Here, we present a tagging strategy for cryoET that precisely identifies individual protein complexes in tomograms without relying on metal clusters. Our method makes use of DNA origami to produce “molecular signposts” that target molecules of interest, here via fluorescent fusion proteins, providing a platform generally applicable to biological surfaces. We have used DNA origami to construct a “signpost” structure, where the “sign” provides the signal for identification in cryoEM images and the bottom of the post is linked to an RNA aptamer that targets common fluorescent proteins (Shui et al., 2012). The signpost origami tags (SPOTs) are used to identify the proteins of interest in a 3D volume of the sample generated by cryoET.

We designed the signpost tags by using the DNA origami method, which enables robust assembly of large and complex nanostructures. In this technique, a long “scaffold” strand is folded into a designed shape through hybridization to many complementary “staple” strands. The signpost is built from a 7,249-nucleotide scaffold strand (single-stranded M13mp18) hybridized to 238 staple oligonucleotides to form a structure of approximately 5 MDa comprising 96 parallel helices arranged in a honeycomb lattice. Signpost origami nanostructures were folded by thermal annealing and purified by polyethylene glycol (PEG) precipitation followed by molecular weight cut-off filtration (full protocols provided in STAR methods). Five mM Mg2+ was maintained in all subsequent preparations to retain proper folding of the nanostructures. The structure of the signpost origami was first verified by negative-stain electron microscopy. Nanostructures were subsequently imaged in vitrified cell lysate by cryoEM to confirm that the contrast of the structure was sufficient to allow it to be identified in crowded biological environments. In projection images, SPOTs are easily identified by the contrast of the repeating stripe patterns generated by the overlap of aligned DNA helices. In tomograms, details to the level of individual DNA helices were visible and the overall shape of the SPOTs was clearly recognizable, and there was sufficient contrast to orient the sub-volume averaging structure by eye. SPOTs have higher contrast than the surrounding protein and often lipids as a result of the phosphorus in the aligned DNA backbones.

> TAAGTACAACCACAGCATTCCAGAACACGTCAACAAATAAGGAACAAAACTCGTATT;> AAGCCAGAATGCCCTTTTAACTGAGGTTTAA;> TCATAACCCGTCGGATGTAGATG;> CAGAGGCCCATCAATATGAGTTTTTATA;> TTGTATCGGATTTTCATAGTTAGCGTAAACCCTCATAGGTGT;> GGAAGCAAACTCCATTGAGTTAAGCC;> TCAGATGATGGCAATTATCATATTTACAAAGTCTTTC;> GAGTAGATTTAGATAACCTGTTTA;> TTTTTGAGAGATATTTAGG;> CATCACGCAAATGCCGGAGAAGG;> ATATATCGGTTATGCGTGGGCGATGGTTGTTGTCATTGTCGGCGCAACTATCGGTATCAAGCTGTTTAAGAAATTCACCTCGAAAGCAAGCTGATAAACCGATACAATTAAAGGCTCCTTTTGGAGCCTTTTTTTTGGAGATTTTCAACGTGAAAAAATTATTATTCGCAATTCCTTTAGTTGTTCCTTTCTATTCTCACTCCGCTGAAACTGTTGAAAGTTGTTTAGCAAAATCCCATACAGAAAATTCATTTACTAACGTCTGGAAAGACGACAAAACTTTAGATCGTTACGCTAACTATGAGGGCTGTCTGTGGAATGCTACAGGCGTTGTAGTTTGTACTGGTGACGAAACTCAGTGTTACGGTACATGGGTTCCTATTGGGCTTGCTATCCCTGAAAATGAGGGTGGTGGCTCTGAGGGTGGCGGTTCTGAGGGTGGCGGTTCTGAGGGTGGCGGTACTAAACCTCCTGAGTACGGTGATACACCTATTCCGGGCTATACTTATATCAACCCTCTCGACGGCACTTATCCGCCTGGTACTGAGCAAAACCCCGCTAATCCTAATCCTTCTCTTGAGGAGTCTCAGCCTCTTAATACTTTCATGTTTCAGAATAATAGGTTCCGAAATAGGCAGGGGGCATTAACTGTTTATACGGGCACTGTTACTCAAGGCACTGACCCCGTTAAAACTTATTACCAGTACACTCCTGTATCATCAAAAGCCATGTATGACGCTTACTGGAACGGTAAATTCAGAGACTGCGCTTTCCATTCTGGCTTTAATGAGGATTTATTTGTTTGTGAATATCAAGGCCAATCGTCTGACCTGCCTCAACCTCCTGTCAATGCTGGCGGCGGCTCTGGTGGTGGTTCTGGTGGCGGCTCTGAGGGTGGTGGCTCTGAGGGTGGCGGTTCTGAGGGTGGCGGCTCTGAGGGAGGCGGTTCCGGTGGTGGCTCTGGTTCCGGTGATTTTGATTATGAAAAGATGGCAAACGCTAATAAGGGGGCTATGACCGAAAATGCCGATGAAAACGCGCTACAGTCTGACGCTAAAGGCAAACTTGATTCTGTCGCTACTGATTACGGTGCTGCTATCGATGGTTTCATTGGTGACGTTTCCGGCCTTGCTAATGGTAATGGTGCTACTGGTGATTTTGCTGGCTCTAATTCCCAAATGGCTCAAGTCGGTGACGGTGATAATTCACCTTTAATGAATAATTTCCGTCAATATTTACCTTCCCTCCCTCAATCGGTTGAATGTCGCCCTTTTGTCTTTGGCGCTGGTAAACCATATGAATTTTCTATTGATTGTGACAAAATAAACTTATTCCGTGGTGTCTTTGCGTTTCTTTTATATGTTGCCACCTTTATGTATGTATTTTCTACGTTTGCTAACATACTGCGTAATAAGGAGTCTTAATCATGCCAGTTCTTTTGGGTATTCCGTTATTATTGCGTTTCCTCGGTTTCCTTCTGGTAACTTTGTTCGGCTATCTGCTTACTTTTCTTAAAAAGGGCTTCGGTAAGATAGCTATTGCTATTTCATTGTTTCTTGCTCTTATTATTGGGCTTAACTCAATTCTTGTGGGTTATCTCTCTGATATTAGCGCTCAATTACCCTCTGACTTTGTTCAGGGTGTTCAGTTAATTCTCCCGTCTAATGCGCTTCCCTGTTTTTATGTTATTCTCTCTGTAAAGGCTGCTATTTTCATTTTTGACGTTAAACAAAAAATCGTTTCTTATTTGGATTGGGATAAATAATATGGCTGTTTATTTTGTAACTGGCAAATTAGGCTCTGGAAAGACGCTCGTTAGCGTTGGTAAGATTCAGGATAAAATTGTAGCTGGGTGCAAAATAGCAACTAATCTTGATTTAAGGCTTCAAAACCTCCCGCAAGTCGGGAGGTTCGCTAAAACGCCTCGCGTTCTTAGAATACCGGATAAGCCTTCTATATCTGATTTGCTTGCTATTGGGCGCGGTAATGATTCCTACGATGAAAATAAAAACGGCTTGCTTGTTCTCGATGAGTGCGGTACTTGGTTTAATACCCGTTCTTGGAATGATAAGGAAAGACAGCCGATTATTGATTGGTTTCTACATGCTCGTAAATTAGGATGGGATATTATTTTTCTTGTTCAGGACTTATCTATTGTTGATAAACAGGCGCGTTCTGCATTAGCTGAACATGTTGTTTATTGTCGTCGTCTGGACAGAATTACTTTACCTTTTGTCGGTACTTTATATTCTCTTATTACTGGCTCGAAAATGCCTCTGCCTAAATTACATGTTGGCGTTGTTAAATATGGCGATTCTCAATTAAGCCCTACTGTTGAGCGTTGGCTTTATACTGGTAAGAATTTGTATAACGCATATGATACTAAACAGGCTTTTTCTAGTAATTATGATTCCGGTGTTTATTCTTATTTAACGCCTTATTTATCACACGGTCGGTATTTCAAACCATTAAATTTAGGTCAGAAGATGAAATTAACTAAAATATATTTGAAAAAGTTTTCTCGCGTTCTTTGTCTTGCGATTGGATTTGCATCAGCATTTACATATAGTTATATAACCCAACCTAAGCCGGAGGTTAAAAAGGTAGTCTCTCAGACCTATGATTTTGATAAATTCACTATTGACTCTTCTCAGCGTCTTAATCTAAGCTATCGCTATGTTTTCAAGGATTCTAAGGGAAAATTAATTAATAGCGACGATTTACAGAAGCAAGGTTATTCACTCACATATATTGATTTATGTACTGTTTCCATTAAAAAAGGTAATTCAAATGAAATTGTTAAATGTAATTAATTTTGTTTTCTTGATGTTTGTTTCATCATCTTCTTTTGCTCAGGTAATTGAAATGAATAATTCGCCTCTGCGCGATTTTGTAACTTGGTATTCAAAGCAATCAGGCGAATCCGTTATTGTTTCTCCCGATGTAAAAGGTACTGTTACTGTATATTCATCTGACGTTAAACCTGAAAATCTACGCAATTTCTTTATTTCTGTTTTACGTGCAAATAATTTTGATATGGTAGGTTCTAACCCTTCCATTATTCAGAAGTATAATCCAAACAATCAGGATTATATTGATGAATTGCCATCATCTGATAATCAGGAATATGATGATAATTCCGCTCCTTCTGGTGGTTTCTTTGTTCCGCAAAATGATAATGTTACTCAAACTTTTAAAATTAATAACGTTCGGGCAAAGGATTTAATACGAGTTGTCGAATTGTTTGTAAAGTCTAATACTTCTAAATCCTCAAATGTATTATCTATTGACGGCTCTAATCTATTAGTTGTTAGTGCTCCTAAAGATATTTTAGATAACCTTCCTCAATTCCTTTCAACTGTTGATTTGCCAACTGACCAGATATTGATTGAGGGTTTGATATTTGAGGTTCAGCAAGGTGATGCTTTAGATTTTTCATTTGCTGCTGGCTCTCAGCGTGGCACTGTTGCAGGCGGTGTTAATACTGACCGCCTCACCTCTGTTTTATCTTCTGCTGGTGGTTCGTTCGGTATTTTTAATGGCGATGTTTTAGGGCTATCAGTTCGCGCATTAAAGACTAATAGCCATTCAAAAATATTGTCTGTGCCACGTATTCTTACGCTTTCAGGTCAGAAGGGTTCTATCTCTGTTGGCCAGAATGTCCCTTTTATTACTGGTCGTGTGACTGGTGAATCTGCCAATGTAAATAATCCATTTCAGACGATTGAGCGTCAAAATGTAGGTATTTCCATGAGCGTTTTTCCTGTTGCAATGGCTGGCGGTAATATTGTTCTGGATATTACCAGCAAGGCCGATAGTTTGAGTTCTTCTACTCAGGCAAGTGATGTTATTACTAATCAAAGAAGTATTGCTACAACGGTTAATTTGCGTGATGGACAGACTCTTTTACTCGGTGGCCTCACTGATTATAAAAACACTTCTCAGGATTCTGGCGTACCGTTCCTGTCTAAAATCCCTTTAATCGGCCTCCTGTTTAGCTCCCGCTCTGATTCTAACGAGGAAAGCACGTTATACGTGCTCGTCAAAGCAACCATAGTACGCGCCCTGTAGCGGCGCATTAAGCGCGGCGGGTGTGGTGGTTACGCGCAGCGTGACCGCTACACTTGCCAGCGCCCTAGCGCCCGCTCCTTTCGCTTTCTTCCCTTCCTTTCTCGCCACGTTCGCCGGCTTTCCCCGTCAAGCTCTAAATCGGGGGCTCCCTTTAGGGTTCCGATTTAGTGCTTTACGGCACCTCGACCCCAAAAAACTTGATTTGGGTGATGGTTCACGTAGTGGGCCATCGCCTGATAGACGGTTTTTCGCCCTTTGACGTTGGAGTCCACGTTCTTTAATAGTGGACTCTTGTTCCAAACTGGAACAACACTCAACCCTATCTCGGGCTATTCTTTTGATTTATAAGGGATTTTGCCGATTTCGGAACCACCATCAAACAGGATTTTCGCCTGCTGGGGCAAACCAGCGTGGACCGCTTGCTGCAACTCTCTCAGGGCCAGGCGGTGAAGGGCAATCAGCTGTTGCCCGTCTCACTGGTGAAAAGAAAAACCACCCTGGCGCCCAATACGCAAACCGCCTCTCCCCGCGCGTTGGCCGATTCATTAATGCAGCTGGCACGACAGGTTTCCCGACTGGAAAGCGGGCAGTGAGCGCAACGCAATTAATGTGAGTTAGCTCACTCATTAGGCACCCCAGGCTTTACACTTTATGCTTCCGGCTCGTATGTTGTGTGGAATTGTGAGCGGATAACAATTTCACACAGGAAACAGCTATGACCATGATTACGAATTCGAGCTCGGTACCCGGGGATCCTCTAGAGTCGACCTGCAGGCATGCAAGCTTGGCACTGGCCGTCGTTTTACAACGTCGTGACTGGGAAAACCCTGGCGTTACCCAACTTAATCGCCTTGCAGCACATCCCCCTTTCGCCAGCTGGCGTAATAGCGAAGAGGCCCGCACCGATCGCCCTTCCCAACAGTTGCGCAGCCTGAATGGCGAATGGCGCTTTGCCTGGTTTCCGGCACCAGAAGCGGTGCCGGAAAGCTGGCTGGAGTGCGATCTTCCTGAGGCCGATACTGTCGTCGTCCCCTCAAACTGGCAGATGCACGGTTACGATGCGCCCATCTACACCAACGTGACCTATCCCATTACGGTCAATCCGCCGTTTGTTCCCACGGAGAATCCGACGGGTTGTTACTCGCTCACATTTAATGTTGATGAAAGCTGGCTACAGGAAGGCCAGACGCGAATTATTTTTGATGGCGTTCCTATTGGTTAAAAAATGAGCTGATTTAACAAAAATTTAATGCGAATTTTAACAAAATATTAACGTTTACAATTTAAATATTTGCTTATACAATCTTCCTGTTTTTGGGGCTTTTCTGATTATCAACCGGGGTACATATGATTGACATGCTAGTTTTACGATTACCGTTCATCGATTCTCTTGTTTGCTCCAGACTCTCAGGCAATGACCTGATAGCCTTTGTAGATCTCTCAAAAATAGCTACCCTCTCCGGCATTAATTTATCAGCTAGAACGGTTGAATATCATATTGATGGTGATTTGACTGTCTCCGGCCTTTCTCACCCTTTTGAATCTTTACCTACACATTACTCAGGCATTGCATTTAAAATATATGAGGGTTCTAAAAATTTTTATCCTTGCGTTGAAATAAAGGCTTCTCCCGCAAAAGTATTACAGGGTCATAATGTTTTTGGTACAACCGATTTAGCTTTATGCTCTGAGGCTTTATTGCTTAATTTTGCTAATTCTTTGCCTTGCCTGTATGATTTATTGGATGTTAATGCTACTACTATTAGTAGAATTGATGCCACCTTTTCAGCTCGCGCCCCAAATGAAAATATAGCTAAACAGGTTATTGACCATTTGCGAAATGTATCTAATGGTCAAACTAAATCTACTCGTTCGCAGAATTGGGAATCAACTGTTATATGGAATGAAACTTCCAGACACCGTACTTTAGTTGCATATTTAAAACATGTTGAGCTACAGCATTATATTCAGCAATTAAGCTCTAAGCCATCCGCAAAAATGACCTCTTATCAAAAGGAGCAATTAAAGGTACTCTCTAATCCTGACCTGTTGGAGTTTGCTTCCGGTCTGGTTCGCTTTGAAGCTCGAATTAAAACGCGATATTTGAAGTCTTTCGGGCTTCCTCTTAATCTTTTTGATGCAATCCGCTTTGCTTCTGACTATAATAGTCAGGGTAAAGACCTGATTTTTGATTTATGGTCATTCTCGTTTTCTGAACTGTTTAAAGCATTTGAGGGGGATTCAATGAATATTTATGACGATTCCGCAGTATTGGACGCTATCCAGTCTAAACATTTTACTATTACCCCCTCTGGCAAAACTTCTTTTGCAAAAGCCTCTCGCTATTTTGGTTTTTATCGTCGTCTGGTAAACGAGGGTTATGATAGTGTTGCTCTTACTATGCCTCGTAATTCCTTTTGGCGTTATGTATCTGCATTAGTTGAATGTGGTATTCCTAAATCTCAACTGATGAATCTTTCTACCTGTAATAATGTTGTTCCGTTAGTTCGTTTTATTAACGTAGATTTTTCTTCCCAACGTCCTGACTGGTATAATGAGCCAGTTCTTAAAATCGCATAAGGTAATTCACAATGATTAAAGTTGAAATTAAACCATCTCAAGCCCAATTTACTACTCGTTCTGGTGTTTCTCGTCAGGGCAAGCCTTATTCACTGAATGAGCAGCTTTGTTACGTTGATTTGGGTAATGAATATCCGGTTCTTGTCAAGATTACTCTTGATGAAGGTCAGCCAGCCTATGCGCCTGGTCTGTACACCGTTCATCTGTCCTCTTTCAAAGTTGGTCAGTTCGGTTCCCTTATGATTGACCGTCTGCGCCTCGTTCCGGCTAAGTAACATGGAGCAGGTCGCGGATTTCGACACAATTTATCAGGCGATGATACAAATCTCCGTTGTACTTTGTTTCGCGCTTGGTATAATCGCTGGGGGTCAAAGATGAGTGTTTTAGTGTATTCTTTTGCCTCTTTCGTTTTAGGTTGGTGCCTTCGTAGTGGCATTACGTATTTTACCCGTTTAATGGAAACTTCCTCATGAAAAAGTCTTTAGTCCTCAAAGCCTCTGTAGCCGTTGCTACCCTCGTTCCGATGCTGTCTTTCGCTGCTGAGGGTGACGATCCCGCAAAAGCGGCCTTTAACTCCCTGCAAGCCTCAGCGACCGA;> GACAATATTTTTCGCGAG;> TAATCAGTAGCGACATAGTAAGAGCAAGGCTTTGTTTTGC;> GGGTCAGCGATTATAAAGAGGCAAAAGAAACGGCTATCGTCA;> AAACAAATACAGATAGCC;> AGATTAAGATTGGGTTAT;> ATTAATGCCGAGAGTCTG;> TCGCCCAGCAGGGAGACTTTTCAACATTGAAAGATTCA;> CAATAATTGTACAGGAGTAATCTT;> TTACGCCAGTTTCCCAGT;> TACTTTTCATCGTAGGAATCATTTAGT;> ATTGCCTGGAGAGGCCGTTCTGAGAAAGTAACCGTCACTTGCCTGAGTAGAAGA;> GTTCCGAAATCGGCAAATACTTCTTGATGGTG;> CGAGCCGGAAGCATAAAGGAAAGGACCTTGTAAAGCC;> ACGACGATAAAAGTAAAAT;> CCCGTATAAACTTCTTAAGATATTCAC;> GGCTGACCTAACAAAGCT;> ACCGTAATGGGAAGGGGACGA;> TTGAAAATAGAAACAGTACAAACTACAAATAGGAGATAAGTG;> AAGTAAGAATCCTCTGGCCTTACAGCTTCAGCGAAGGAACGAGGG;> AAGTTCTTAATTGTGTCTGGAAGTATTTTGCAC;> ATAGCAAGCATTTTGAAGGAACCAGCCGCCAGACAGGAGCAGTCTGGCTTTTGA;> GGTCCGATGAACGGTAATCGTAAAATT;> TATAATAAAAGAGTCTGTC;> TAGAACCCTTCTCGTAAGAATACGTGGCACA;> CAGAGGGTCACCAGATTTGTATCATC;> CTATTATCCCGGAAGAGCCACCACCCTCCAGCCCTGCTAAAC;> GACAAGAACAGCCGCCGC;> TGGTTCTCCGTTCAAATAAGATTAAGAGGAAGCC;> CGAATAATAATTAGGATTAGC;> GAGCGCTAGAAACAACTGGCACAAACGTAATAGTGCTTTTTAACCT;> TAAGTTGGGTAACGGACGGCC;> TATAGAAGGCTTATAACCTCCACCGCCTCTCAGAGAGACGATATTA;> CAACATGTACTACAAAGGCTAAGGAGGCCG;> ATCAGTGAGGCCACCGAGATCAA;> TGAGCTAACGTGCCAGCT;> CGTCACCAATGAAACCATAAGAATGCAACGATAGCAGCACCG;> TCAAGAGCCAGGCGACCCATGTACCGTAACACT;> CCAGCGGATATTCATTGTCATTTCTTAGAGTGAGTAACCGAAC;> GGCGCATTAATTAACAAAA;> TCGGTCGCTTAGTAAATTGGGCTGAATTAC;> TTAGACGAATAACACGCCACCCCCTCAGAGCCGCCAC;> GTTATTAATTGCGATGCAAGTTAA;> GCTATATTTTCATCTACTATTGCGCTTTTCCAG;> TTAATTGAGAATCGCCCGCTCAATGAATTAATTGACGAGTG;> GTTGAGTGTTGTTCCGCCA;> TCACATTTGGGGTGCCTAATGAG;> TAGCGTCCAATACTGAGCCAATTAGCGGAATCGTCATA;> CGAGATCCCCCTCAAACGAT;> CCACGCCTTTAGCCATATGGAGCGGAGACTTTACA;> CATCTGCAGGAAGAGCGAACCAGACC;> AAGCATCTTTAATCACCGCCTTAACAATTTTTCAATATATATCTTTAG;> GGAAGCGCAACAGTAACA;> AAATATCTAAACTGGTCAGGTCAGTATTA;> CTGCTCATCCGCAAAAAG;> GAGCAAACACGGTTGATA;> GAGAAGTTATTCAAGTAGCTAGTTTAGACTGGA;> AATTGCGATAGTAGTAGCA;> AGCAAAAGGTAATAACCAAAATAAAGTACAGCTAATGCAGAACGCGC;> TACTGGCGACAATCCGTAA;> CCTCAGAACTAAAAACAG;> TCTGTAAATCGTCGCTATCGTAACCGTG;> CCCTCAGGATACCGAGTAACAGTG;> GAGAGTACCTTTAATTGCTATAATGCATGTGCT;> AACAACTAACATATCAAACAACAGTGCCA;> GTGGAGGCAAAGACGTTGGGAAG;> CTTACTTGAGCCATTTGGG;> CGGTACAGTTTGGAACAAG;> TCGGGAACAACGCGTCGGTTGTACCA;> CATTAAAGGCAGTAGGGC;> TGATACAGGGAAATTATT;> GCTCATTCAGATTCCCGCAACTATCGACTCAGTGCCAAGCTTGCATAAAGG;> CCTTGCTTTAGAATCCTTGAAAAGAGTCAGAAAATCGCAAAG;> ACGTTGGTGAATAGTTAATGCCCCCTTACTCAGCCCTCAG;> ATAAGAGACCCAAAAGGCTTGCCCTGACGAGAAAC;> ACATTTGAGGATTTAGGCCG;> TTAAACCAAGTACGAGAACAA;> ATATCATATGGCTGCGCACGGGGAAAGCCGG;> ATTAAAGGGATTTTAGACAGGAAGAATCCT;> CTGGCCACCCGCCACTGACAGAGA;> AATATTCATTGAGCGCAGACGGTC;> AATCATAAGGGAGCATAGGCT;> ACATCAATCATACAGAACGAGGAGGCTTCGCATAAGTGTCGACTGCTCC;> AGTACATAAACATCAAGACGCAATTACCGAAGGAAAGCGGTTGAGCGCCGACTTGCGGG;> AACTTTCAAAGGAGCATGAAAGTATTAAAGAGGGTGGGATAG;> TTGCGTTTTGTTTACACCA;> CACGACGTTGTAAAACCCAGGGTCTGGCGA;> TTAACATCCAATAAATCATAGCTAAACGGGGAGCGTATTG;> TACAAACTAGCATGTCGCTGGCAGGCGAGA;> AGTCCACTATTAAAATCAG;> GCATTAATGAATCGGCACCTGTC;> TGAGGATGTTACCTTTGAAAGAGGAGTAAGCGT;> ACCGAACGGATTGCATCAAAATCGCGTT;> GAGCCACCACCGGACGACTTGCAACGCTCCTCAAAACTAATA;> ATTTGAATTACCTTTTTACATTTTACCAGA;> ACAGAGGCTTTGAGTAAAACGACCAAGCGGCCGGAAA;> CCCAATCAAATGAAGAACAAAGCTATCTAATAACGTAAAGGTGG;> AATTGAGGAAGGTTCCTTTGCCATTATCTGGAAGGGTAAAACTTACAAACCTGAGC;> AGCATAAACAGGCACATCAATTTTGGGGGAATGGCTAATGCGCGAACTGATAGC;> TACTAGAAACGCCGCGCT;> TTAGAGAACGTGGACTCCA;> GGCGCCAAACAGCTTATATTTTAAAT;> GAGGGAAAAGGGCGTTAAATATACCGACTGCCGTAAAG;> CATACATCTGAATTAGCAATAGTCAGAGAAGAAATATACTTCTGA;> ATTAGCGTTTGCGCCGCTTAATGACATTTAACG;> CGACAGTATCGGAAACCA;> TAGCATACACTTCTTTGACCCCCAGTGCCTTGATAGTTGGCAGGTCCCA;> ATTTGCCAGTCCTGATTA;> GAGCATTCGACAGAAACCTTGGATTTGCGTAGCTGATTGCTTT;> TCAGTGCGGGATACCACATTCAA;> ATCAGAAAATATTTTGCTACGTGAAC;> ACGTGCTCTAGGGCAATCATAAAACAGGTTCAGAATTTACCCTGACTATTA;> ATAAAAGGTTTGAGGCGGGACATT;> CAACTGCTTTAAACAGAAGATTG;> TGAACGGAAGAGCAAATATCATTTGCACGTTAGAACCTACCATAGTTGGGAAGGGC;> CAACTTTAAATGGTCATTTGACCCCATTAACGAACCACCAGCAGAAGATAAAACAG;> CCAGCTTATTCATTGACTC;> GTCGTCTTTGCATCAGACACCAG;> TGTTTTAAATATAATTCTGCGAAC;> GATTAGAAAGTATTAATTATCCATCAATCGTCAGAGAGAAACAATTAATTTAATGGAAAC;> TCCAAGATTAAGCAAAAACGGGTA;> TATAAAATAAGGCGACATT;> TGGTTGCTTTCGGTCACCGTTA;> CACCAGTGAAAGCGGTCC;> TGGTTTACCAATCATAAT;> CTTATGCGATTTTAAGGGCAT;> AAAAGAACAAAAGAATGAAATTACCGTTCCACAGA;> CCACAGAATTTTCATGATATAAGTATAGTCTGAAACCTTTAA;> CCAGCTAATCAAGATACCGCGCCCA;> TCAATCACCTCAGCAGCAAATGAAAA;> AAAACATTATGACCCTGTAATACTTT;> GATAGCAAATATTTAATCAAGTT;> TAATGCGCCGCTACAGCCACACCAAGCCTGACACCGGAGCGCCA;> GACGGGCGGGTGGTTTTTCTTTT;> AATCAAAAATTCGCGTTAAATCAGCTCATTACGTTAAGCCCCAATGTACCCAGAGAAT;> CAGTCAGGAATTAGCAATAAAGCC;> AGAGGCGAACAGCTTTCCGGCACCGCTTCCATTCA;> GAGTTTCGTCACGGAACAACTAAAGGAATTG;> TGCTTTCATTCCATATAACAGTTGTGAATATCAACGTTCATCAAACCAGGC;> TAGAGGATCCCCGGGTACCGAGC;> AGAACCCTCAGATTGCCTGGC;> TGGGTTAATTTGTAAATGCTTAGGCGCTGAGAACATAGATGTGAGTGAATAA;> ACGTCAAAGGGCGAAAGGA;> CCTGAGAGAGATTATTTTTTGACGCGCCAGCCTGGTAA;> TAGTCAGAAGTTGGAATAAG;> TCATCAACTGGCTCAACGGAATCATGAGGCCACTAAACGGAGTAGCACCCACCGACCAGT;> GAATACCAAGAGAAATAGGTAATT;> GGGTAAAATCATAACCCATAACGAATAGATACCAATCAATAATCGGCTG;> TTTAGCGCCGGTATTCTAAGAAC;> GCAGGAAGTACGGCTGAATCCTTTTGAACCCACAAGAAACAGGTCAGGATTA;> AAATTGTAGAAAAGTCCTACATGTTCCGACAAACAGTCAAATCAATTTTCGAGCCAGT;> GACCTAAATAACCCTAAA;> AGCGAAAAACCGTCTATCA;> TCACACGCCGCCCTTCAACCAGTA;> CAATAGAAAAGAAAACATACAGAATACCGATGATGAAACAAATCAATATCGATAGCTT;> TGTAGCGCGTTTTTTCGGTCATAGCCCCCTT;> ACGGATTCGCATTTTCAACACCCTAATAGCACCTCAGA;> CCGCCAGAGGTTTAGTAC;> GCGAGGCGTCAGAGCCTA;> ATCTAAAGCATAGATAAT;> TCTTTCCTCAACTTATTTTATCAT;> TTAAATTTTTGTCTGGCCTTCCTG;> AAGGAAGACCCAAAATTGTAATTTTAACCAATAACGCG;> ACGCTGGCTGAAATGGTTGCAGC;> CAAAGCTGACCAATTAGCCGGAA;> AAAAATCTACGTTAATAAA;> GTACCTTTTACATCGGTGAATAT;> AACCGCCCGATCTAGAATTTTCTGTATGGGTTTATTCGGAAC;> TCGAATTCGTAATCATGGCCGAA;> GCAATGCCCATCATATCCTGAGTA;> AGAAAACTTTTAATCGCAAGACTACAATTTATTTTTCCC;> CGAACGTAGTGTAGGACGAGCACGTATA;> CTCATGGAAATAACGAGCATTTT;> ACACCACTATTTTGCAAATCCTCAAATATAT;> TTAGGAAGAAGCCTGCAAGGATAA;> GGCAAAGCGTCTTCGCTA;> CAAGCCCACGCCTGTCAGCGGAGTGAGAATCTCCAAGACTCC;> AGGTGAGGCGTTGGCAAATCAACAGTTGGCCT;> AAAAATACTAATTTCCTACATACATTGGCAGATTCACCAG;> TTTATTTGAAAAGAATAATTTAGTAAAGCCAAATATTTAACAACGC;> GGGAGCCCCCGATTTAAAATCGGTTAA;> CAGCAGGCAATATTACCTCAATCGTTTTGCCC;> CAACATATAAAATTCATA;> TCAGGAATTACGAGGCAGAATCAAGTTTGC;> GGCTGCGCAACTTCAAAATTAGAGAGAT;> AAAGTACCGAAGGCACCAACCGACTAAAGTTA;> ACACCGCCTGCCCTCAAATCCTGA;> CTGTTTATCAACCCAAAAGTTGAGATACGAACTATTATAC;> AAGAGGAACGCCATCATGAGCGA;> GGCGATGGCCCATTAAAATTCGCA;> CATTGCAACAGGAAAAACG;> CGAAAGACTGGGAACAATCAACATTA;> CTTTAGCAGGTAATTACGTCAGAC;> GCGGGCCCCATTCGCTGGTGCCGGCCTCCAGTTTGTAGGTCACGT;> CGCCACTCAAAAACACCCTCAGAA;> CGCTGAGAGCTGCTGAAAACGAGCATAAACACAGAGAGGGAGAATTTAAGAAAGGA;> ATGTGTACAGACCTGTCGGTAAAG;> ATAACTATATCATCTTCT;> CATCGGAAGAAGCGGGCGTTCCTCGAGCGGGAGCTAAACTCA;> ACTCAAACTATCATAAACAGAACAAG;> TTAATTTACGCAGTATGTTAGTGATTAATCAATTAATCGCGC;> CTAATGCAGATACTCGTTTACCAG;> GATCGGTAAGGGGGTGTAGCTCAACA;> ATCACCGGCCTATTCAGCTTGCTTTCGAAGTAAATAAGTTTT;> AAATATCATAGCTGTTTCCTGTG;> TAAAGTAATTGACGACAGGCCTTG;> TAGCCAGCTTTCAACGGCGGATTG;> TTTTGGGGTCGAGGCGTGT;> CCTGTTTTGATTAGTATATCCAGAACGAAAAT;> CTTATCGAGCTTCAAATCGCACT;> CTATACGTAATGAAGTTTCCATTAAAC;> ATAAATTTTGCGAAACGATTGATGG;> CCGTCGGAGGCTGAAAAAAAGGCTCCAAACAGTTTAGCATT;> CCTAAAACATCGATTAGA;> AATAAGAGAATATAGCGAGACA;> AATGAAAATAATCAGGTCAACGAGAATGACCATA;> CACTGAGCTTGGTAACCAGGCGCGTACTA;> ATAACATTGTAGCAAATCCCTAAGAATAGCCCGAGATAGG;> AACCGAGGAAAAAACAAAATA;> ATAATCCTGATTGTACCAGAATATTTATATCTTACCGGGAGGAATCAGA;> GGGGTTTTGCTCAGTAAAGGATTTTTTCACG;> TGAAATTGTTATCCGCTCGTCTT;> ATTCAAAAGGGTAGCTGATAA;> GTAACAGGTCTGAGAGACA;> GAACAAAGTAACAATTTC;> GCCTGATAAATTCCGATATAT;> TATTAACAATTCCACACAACATA;> CCGGCTGATGTCACAATAAGACAAGGTAAATTCACCGTATTACCATTAGCAAGCGAAAC> M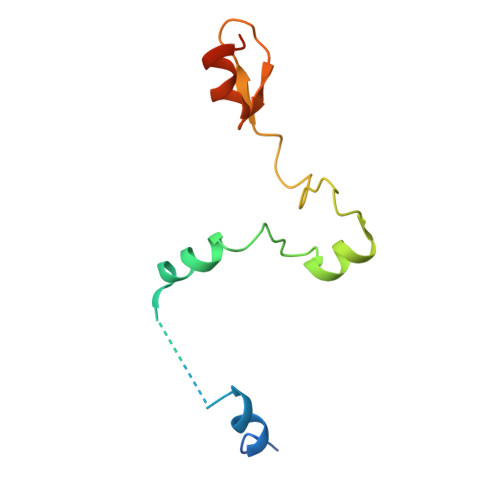RSGDAEIKGIKPKVIEEYSLSQGSGPSNDSWKSLMSSAKDTPLQYDHMNRESLKKYFNPNAQLIEDPLDKPIQYRVCEKCGKPLALTAIVDHLENHCAGASGK> MEFKKVAKETAITLQSYLTYQAVRLISQQLSETNPGQAIWLGEFSKRHPIQESDLYLEAMMLENKELVLRILTVRENLAEGVLEFLPEMVLSQIKQSNGNHRRSLLERLTQVDSSSTDQTEPNPGESD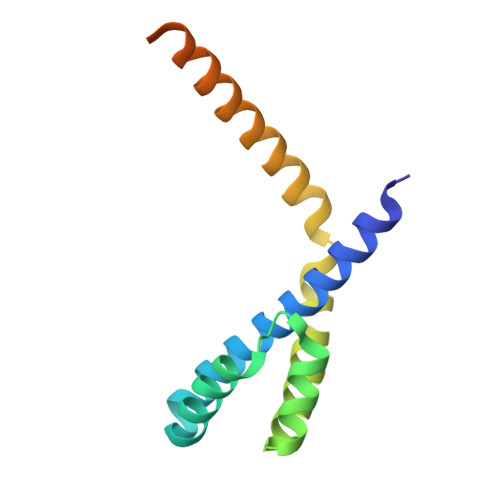TSEDSE> MENTENSVDSKSIKNLEPKIIHGSESMDSGISLDNSYKMDYPEMGLCIIINNKNFHKSTGMTSRSGTDVDAANLRETFRNLKYEVRNKNDLTREEIVELMRDVSKEDHSKRSSFVCVLLSHGEEGIIFGTNGPVDLKK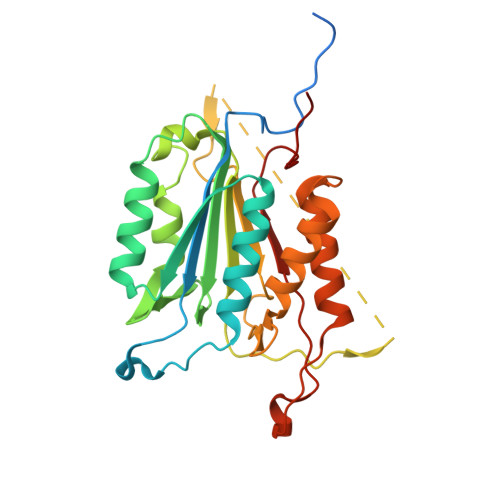ITNFFRGDRCRSLTGKPKLFIIQACRGTELDCGIETDSGVDDDMACHKIPVEADFLYAYSTAPGYYSWRNSKDGSWFIQSLCAMLKQYADKLEFMHILTRVNRKVATEFESFSFDATFHAKKQIPCIFSMLTKELYFYHLH> TLKLCSPEEFTRLCREKTQEIYPIKEANGRTRKALIICNTEFKHLSLRYGANFDIIGMKGLLEDLGYDVVVKEELTAEGMESEMKDFAALS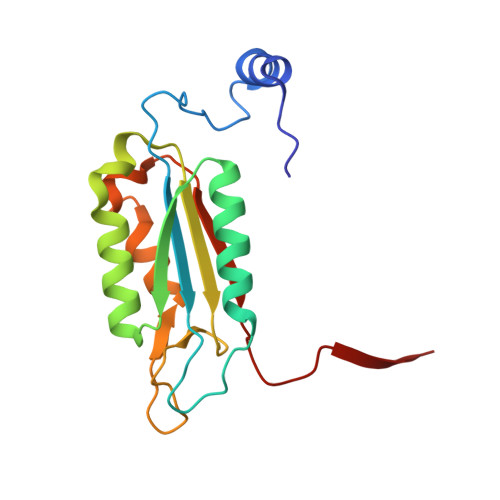EHQTSDSTFLVLMSHGTLHGICGTMHSEKTPDVLQYDTIYQIFNNCHCPGLRDKPKVIIVQAARGGNSGEMWIR~{N}-[4-(4-methylpiperazin-1-yl)phenyl]-4-(2-pyridin-3-yl-6,7-dihydro-4~{H}-pyrazolo[5,1-c][1,4]oxazin-3-yl)pyrimidin-2-amine | C26 H28 N8 O | 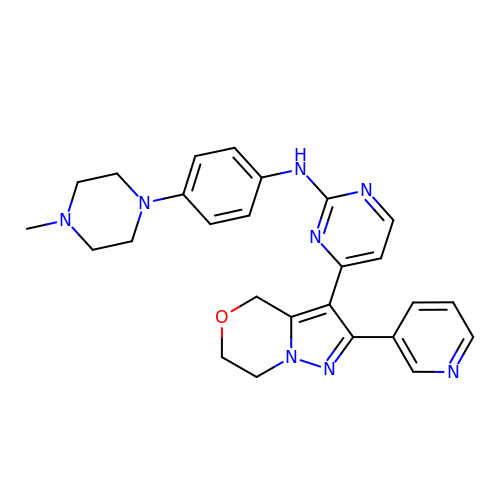OCSGNUMYNBZDDW-UHFFFAOYSA-N> MGSSHHHHHHSSENLYFQ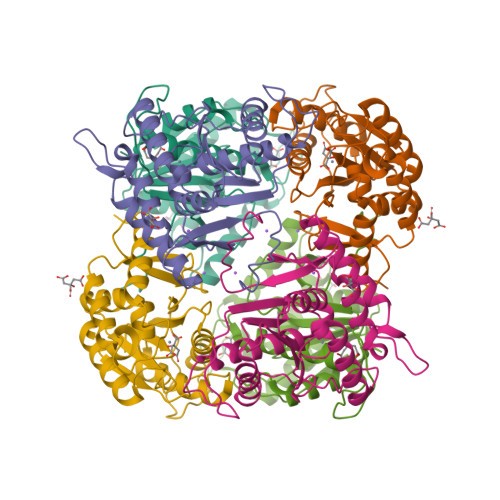GHMYNADVLAFGAHSDDVEIGMGGTIAKFVKQEKKVMICDLTEAELSSNGTVSLRKEEAAEAARILGADKRIQLTLPDRGLIMSDQAIRSIVTVIRICRPKAVFMPYKKDRHPDHGNAAALVEEAIFSAGIHKYKDEKSLPAHKVSKVYYYMINGFHQPDFVIDISDTIEAKKRSLNAYKSQFIPSKDSVSTPLTNGYIEIVEAREKLYGKEAGVEYAEGFFSKRMLMLDHDVLGGEQ> DSKTPADWIDSD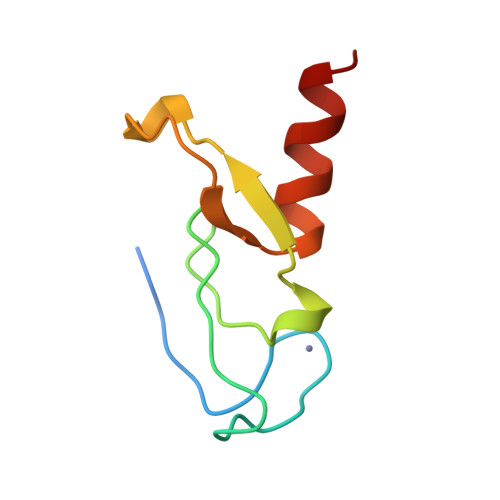ACMICSKKFSLLNRKHHCRSCGGVFCQEHSSNSIPLPDLGIYEPVRVCDSCFEDYEFIVTD> MSTRTRNILIIVGALIISIASRFFLYTGPPHVEVAAEVIFDGIPGFPITNSFVVAIIIDIFVIALAVAATRNLQMVPRGLQNVMEFILESLYNLFRNINAKYVATAFPLVATIFLFVLFGNWFGLLPGVGSIGVCHEKKEEHAVVDERLALAAPAAPLSSVAAAEGEEIHDTCAAQGKKLVPLFRAPAADLNFTFAIAVISFVFIEYWGF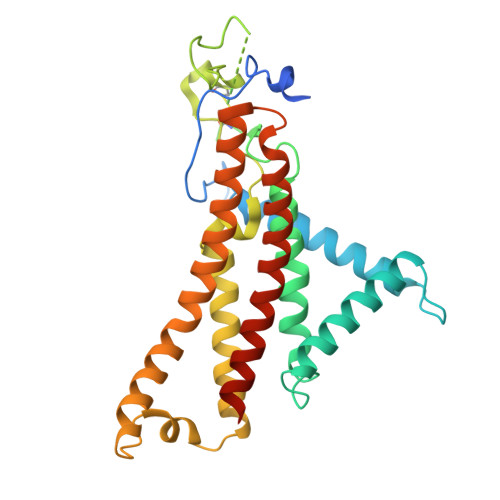RALGPGYLKKFFNTNGIMSFVGIIEFISELVKPFALAFRLFGNIFAGEVLLVVMAFLVPLLLPLPFYGFEVFVGFIQALIFALLTYAFLNIAVTGHDEEHAH>[2x]QLIFDDC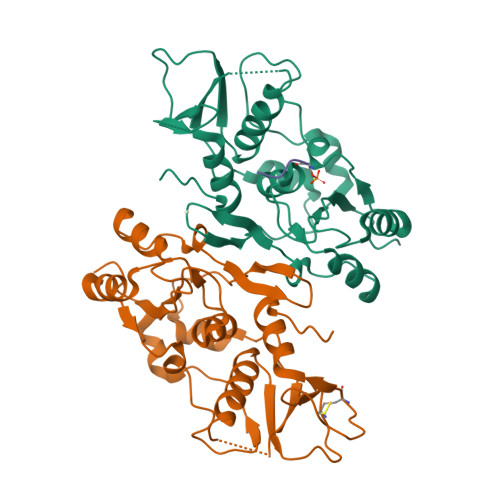VFAFSGPVHEDAYDRSALETVVQDHGGLVLDTGLRPLFNDPFKSKQKKLRHLKPQKRSKSWNQAFVVSDTFSRKVKYLEALAFNIPCVHPQFIKQCLKMNRVVDFSPYLLASGYSHRLDCTLSQRIEPFDTTDSLYDRLLARKGPLFGKKILFIIPEAKSWQKKIENTEQGQKALAHVYHALALGADVEIRPNVAHLECDLILTMDGNIVDETNCPVVDPEWIVECLISQSDIST;> SQEL>GPSSTVTIEYFNQKKEMTKTLEEITRDFEKENPKIKVKVVNVPNAGEVLKTRVLAGDVPDVVNIYPQSIELQEWAKAGVFEDLSNKDYLKRVKNGYAEKYAVNEKVYNVPFTANAYGIYYNKDKFEELGLKVPETWDEFEQLVKDIVAKGQTPFGIAGADAWTLNGYNQLAFATATGGGKEANQYLRYSQPNAIKLSDPIMKDDIKVMDILRINGSKQKNWEGAGYTDVIGAFARGDVLMTPNGSWAITAINEQKPNFKIGTFMIPGKEKGQSLTVGAGDLAWSISATTKHPKEANAFVEYMT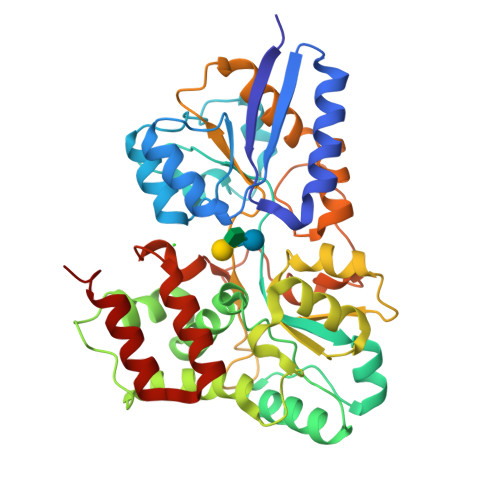RPEVMQKYYDVDGSPTAIEGVKQAGEDSPLAGMTEYAFTDRHLVWLQQYWTSEADFHTLTMNYVLTGDKQGMVNDLNAFFNPMKM[2x]PYRIDIN-4-YLMETHANOL 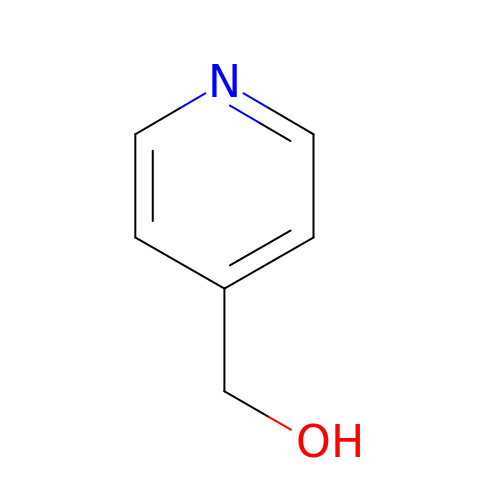| C6 H7 N O | PTMBWNZJOQBTBK-UHFFFAOYSA-N>[3x]QGTTSSATTSQTGNTNTAVIDQVGGLNNSAEASQAGDGNVATVTQAEGMDNAVYIDQVGLTNTATVLQEGGLDNDADVDQDGDLNVAYIWQNLGEDNDADIDQDGTLNDAAIEQDGGEDNDADIDQDGSENAAYVGQTGGEDNDADIDQDGTFNNA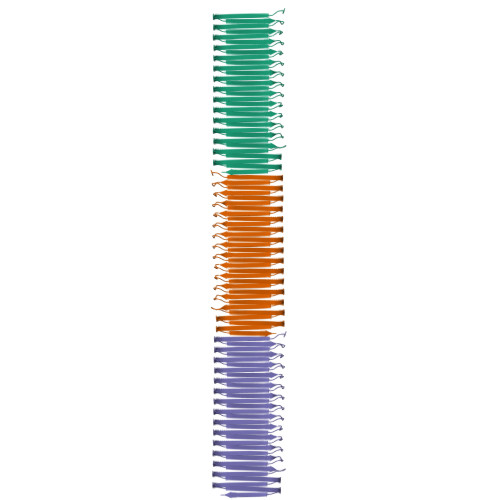YIGQFGGEDNEADLDQDGDANYAAILQDGGEDNDADIDQDGTNNWAETNQIQGNDNDVEVDQDGSDNIAEVWQMHGEDNEANVDQDGDLNNAYILQEGGMNNLADVHQNGVSNTAEIYQYGGMDNEAYLIQDGDMHTGVITQSGDGANYAELNQMGLMNTGSITQDGMGNSAITSQGGSMNMSTVTQSGTGNISLVNQHGGHHHHHH> THVDLGLASANVDFAFSLYKQLVLKAPDKNVIFSPLSISTALAFLSLGAHNTTLTEILKGLKFNLTETSEAEIHQSFQHLLRTLNQSSDELQLSMGNAMFVKEQLSLLDR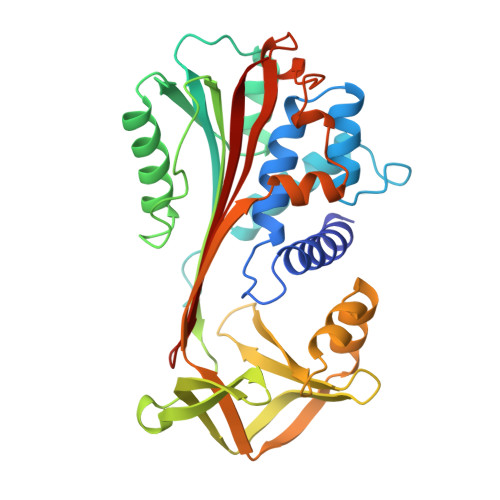FTEDAKRLYGSEAFATDFQDSAAAKKLINDYVKNGTRGKITDLIKDLDSQTMMVLVNYIFFKAKWEMPFDPQDTHQSRFYLSKKKWVMVPMMSLHHLTIPYFRDEELSCTVVELKYTGNASALFILPDQDKMEEVEAMLLPETLKRWRDSLEFREIGELYLPKFSISRDYNLNDILLQLGIEEAFTSKADLSGITGARNLAVSQVVHKAVLDVFEEGTEASRATAVKITLL>[16x]MFGRKKGDVIDAGAELERAEQERIEGEYGASELASERRPHTPGARTLLMVLLCVIAVVLVTLSYKAYKVRGVVEDDDAQPQQVVRQVIPGYTPRPIRPEPENVPEPPQPTTSVPAIQPAPVTQPVRPQPTGPREKTPYELARERMLRSGLTAGSGGGEDLPRPQGGDVPAGGLMGGGGGGGELAEKLQPMRLSGSSAGRLGNRDMLITQGTQLDCVLETRLVTTQPGMTTCHLTRDVYSTSGRVVLLDRGSKVVGFYQGGLRQGQARIFVQWSRIETPSGVVINLDSPGTGPLGEAGLGGWIDRHFWERFGGAIMISLIGDLGDWASRQGSRQGDNSIQFSNTANGVESAAAEALRNSINIPPTLYKNQGERVNILVARDLDFSDVYSLESIPTK;>[16x]MKKLAIVALLASLHAVPALALDVPSSSRYDHRIRYVTYNPADVVQVDTVLGVATHIMLEEGEQYLTHAFGDSEAYAFARKGRHIFIKPQAELANTNLIVVTDRRSYKFRLQMRNDRNGAMYELAFRYPDTQARQTREANARAAVEAAFEQRVGAYYNLKYMMSGDKDIAPVNAWDDGRFTYFKFSANADLPSIYFVDAEGNESLVPRTTVGSSNNIIAVHKVNPKWMIRLGNRALAIFNEAYDPNGVPNDTGTASPAVRRVNKGGN;>MKTIIFAILMTGLLSACASAPKPKQPSDFNREPVNKTVPVEIQRGAL[14x]

Conjugative type IV secretion systems (T4SS) mediate bacterial conjugation, a process that enables the unidirectional exchange of genetic materials between a donor and a recipient bacterial cell. Bacterial conjugation is the primary means by which antibiotic resistance genes spread among bacterial populations. The recent cryo-electron microscopy (cryo-EM) structure of the conjugative Type 4 Secretion System (T4SS) encoded by the plasmid R388 revealed that the remaining VirB proteins form a large assembly organised into four sub-complexes: the outer membrane core complex (OMCC), the stalk, the arches and the inner membrane complex (IMC). Previously, we solved the cryo-electron microscopy (cryo-EM) structure of a conjugative T4SS. In this article, based on additional data, we present a more complete T4SS cryo-EM structure than that published earlier.

Unsymmetrised C1 maps for the entire OMCCs are obtainable, however, they are often of insufficient resolution to derive important structural features such as the TrwF/VirB9 linker sequence between the two layers or to derive detailed information on the symmetry mismatch. In this study, thanks to a larger dataset, we were able to achieve high resolution without imposing any symmetry constraints (Fig. EV1), enabling a more in-depth investigation of the OMCC. In this map, the two additional I-layer binary complexes of TrwF/VirB9NTD and TrwE/VirB10NTD are inserted in diametrically opposite locations. Clear density is seen for 14 linker sequences (residues 128 to 150) between the two domains of TrwF/VirB9, which we can now confirm is mostly α-helical. As anticipated, the biggest impact of domain insertion in the I-layer is observed in this linker helix. When the angle it makes relative to a vertical axis is measured, a pattern can be seen, with the largest angles observed on each side of the insertion (see complexes 2 and 10 or 8 and 16 in Fig. 2A). The angle tappers off the further the complex is from both insertions (see complexes 4 and 12 in the same Figure panels). Clearly, linker helix flexibility is crucial to accommodate complex insertion in the I-layer.>MPPTPTAAAAGAAVAAASAAEQAAFRLVGHRNFVRFNPRSDRFHTLAFHHVELWCADAASAAGRFSFGLGAPLAARSDLSTGNSAHASLLLRSGSLSFLFTAPYAHGADAATAALPSFSAAAARRFAADHGLAVRAVALRVADAEDAFRASVAAGARPAFGPVDLGRGFRLAEVELYGDVVLRYVSYPDGAAGEPFLPGFEGVASPGAADYGLSRFDHIVGNVPELAPAAAYFAGFTGFHEFAEFTTEDVGTAESGLNSMVLANNSENVLLPLNEPVHGTKRRSQIQTFLDHHGGPGVQHMALASDDVLRTLREMQARSAMGGFEFMAPPTSDYYDGVRR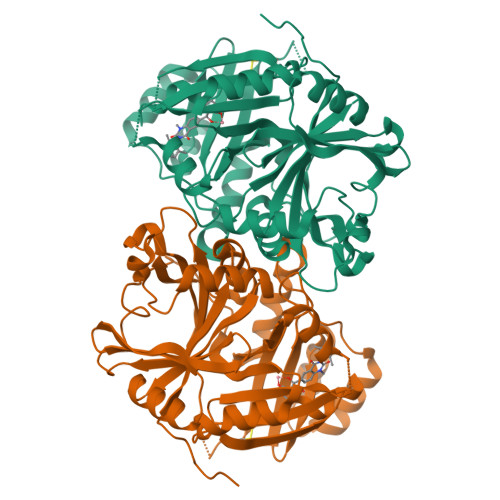RAGDVLTEAQIKECQELGVLVDRDDQGVLLQIFTKPVGDRPTLFLEIIQRIGCMERDEKGQEYQKGGCGGFGKGNFSQLFKSIEDYEKSLEAKQAAAAAAAQGS[4x]(4~{S})-5-[4-[dibutyl-[4-(2-ethyl-2-oxidanyl-butoxy)-3-methyl-phenyl]silyl]-2-methyl-phenoxy]-4-oxidanyl-pentanoic 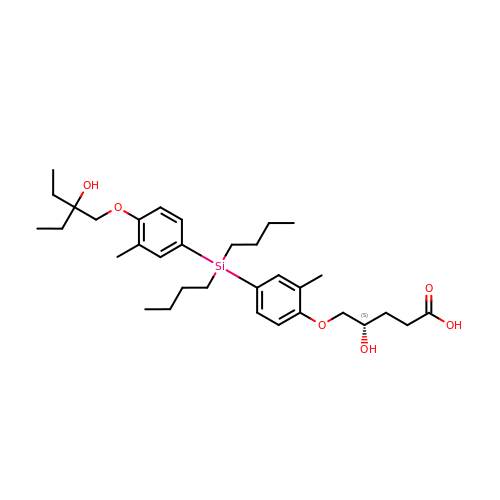acid | C33 H52 O6 Si | VIAQTQKQQPBVMW-MHZLTWQESA-N> SPDFLKLFLNHTTMHGQPPTFDMFSRFCFPSDPERSLASIVLQKLPQMGSPGDPTSLLVDFADTLIDLWHQCLSERYYGPIYHLVSLLLYTLDLNAVEVAPHILSSLIPVCATTCRLVALPRLNSADGDLSGHPDAVVRQLCLNIDVTQCLSVLYLAASGCLPQPLQNPTSSDQPQDTPQL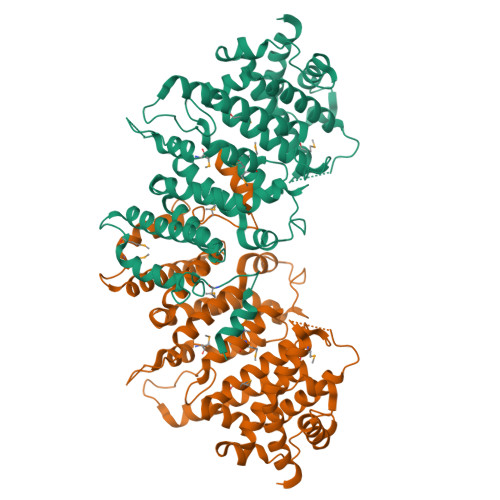EFWKTMELDFVLTMLSPKNPEEDWSAMMILLRTSVAPHSIGPIPSSATNSTNRRSEAKNADAVAATLIDCVSSFLCEPPKWATPRSAKEIAARLAALRTLMAFATGHFGARQIAESDVAIPRLVTVLCWALDRLYDSDLPLSPEPQAGAGRPPDERGDSMELDHPNVESAGGMEAHGTSEGLTDVSAEVTDAAPDSMSLLHQIIAQGTRLLHFLVTDHRTSDAANISTKLAASHGGSQRYFLTLARLNFAEEDLVLEAGIDAETVELAHELLELAVTPDEGDEISEMFD>[2x]MENTENSVASKSIKNLEPKIIHGSESMASGISLDNSYKMDYPEMGLCIIINNKNFHKSTGMTSRSGTDVDAANLRETFRNLKYEVRNKNDLTREEIVELMRDVSKEDHSKRSSFVCVLLSHGEEGIIFGTNGPVDLKKITNFFRGDRCRSLDGKPKLFIIQACRGTELDCGIETD;>SGVDDDMACHKIPVEADFLYAYSTAPGYYSWRNSK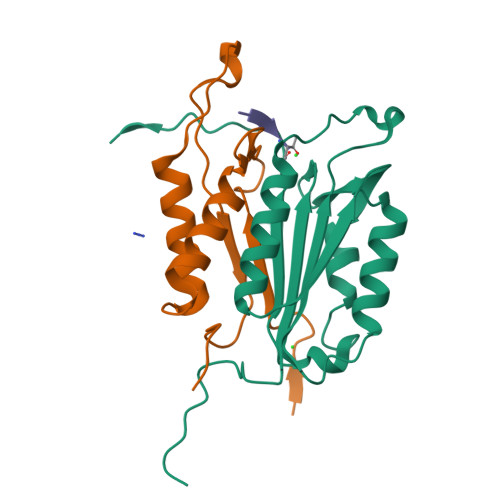DGSWFIQSLCAMLKQYADKLEFMHILTRVNRKVATEFESFSFDATFHAKKQIPCIVSMLTKELYFYHH[2x]> TGRPEWIWLALGTALMGLGTLYFLVKGMGVSDPDAKKFYAITTLVPAIAFTMYLSMLLGYGLTMVPFGGEQNPIYWARYADWLFTTPLLLLNLALLVDADQGTILALVGADGIMIGTGLVGALTKVYSYRFVWWAISTAAMLYILYVLFNVTVVLWSAYPVVWLIGSEGAGIVPLNIETLLFMVL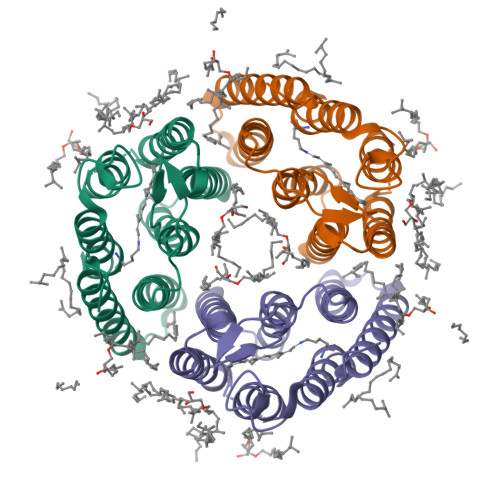DVSAKVGFGLI>[2x]KDTIALVVSTLNNPFFVSLKDGAQKEADKLGYNLVVLDSQNNPAKELANVQDLTVRGTKILLINPTRSDAVGNAVKMANQANIPVITLDRQATKGEVVSHIASDNVLGGKIAGDYIAKKAGEGAKVIELQGIAGTSAARERGEGFQQAVAAHKFNVLASQPADFDRIKGLNVMQNLLTAHPDVQAVFAQNDEMALGALRALQTAGKSDVMVVGFDGTPDGEKAVNDG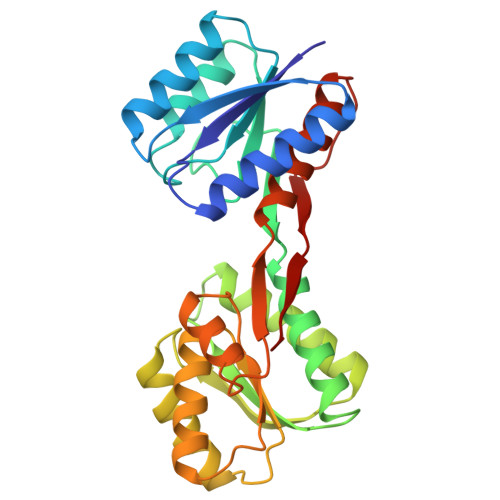KLAATIAQLPDQIGAKGVETADKVLKGEKVQAKYPVDLKLVVKQ> MRLSYEALEWRTPIENSTEPVSLPPPPPFFGQERAREALELAIRGGFHAYLVGPPSLGKHEALLAYLSTQSVETPPDLLYVPLSERKVAVLTLPSGQEIHLAEAVEGLLLEVNRLDELFRQGSFLREKTQLEARFKEAREQQLEALRREAQEAGFALSTNGERLELTGPGPVPAELSARLEEVTLGSLAASAELEVALRRLRRDWALHYLNNRFEPLFQRFPQARAYLEALRARLARYAETGEPLDPAQWRPNLLTSSSSGTPPPIVYEPYATAPRLFGRLDYLVDRGVWSTNVSLIRPGAVHRAQGGYLILDALSLKREGTWEAFKRALRNGQVEPVTEPQAPAGLEVEPFPIQMQVILVGTPEAFEGLEEDPAFSELFRIRAEFSPTLPASPENCTALGGWLLAQGFQLTQGGLTRLYDEARRMAEQRDRMDARLVEIRALAEEAAVLGGGLL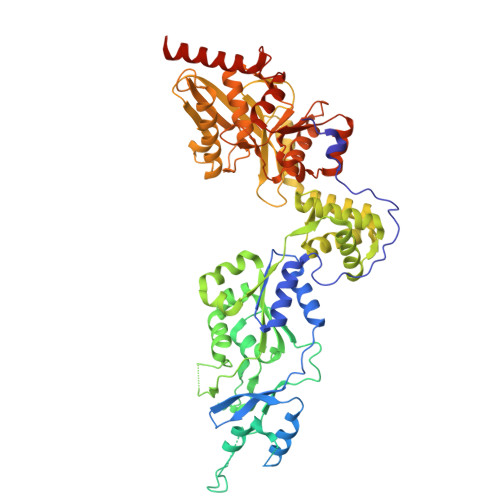TAESVEQAIAAREHRSFLSEEEFLRAVQEGVIRLRTTGRAVGEVNSLVVVEAAPYWGRPARLTARAAPGRDHLISIDREAGLGGQIFHKAVLTLAGYLRSRYIEHGSLPVTISLAFEQNYVSIEGDAAGLAELVAALSAIGNLPLRQDLAVTGAVDQTGKVLAVGAINAKVEGFFRVCKALGLSGTQGVILPEANLANLTLRAEVLEAVRAGQFHIYAVETAEQALEILAGARMEGFRGLQEKIRAGLEAFARLEEGHDKEDREKLAAALEHHHHHH>QTAPKTFTHPDTGIVFNTWSASDSQTKGGFTVGMALPSNALTTDATEFIGYLECSSAKNGANSGWCGVSLRGAMTNNLLITAWPSDGEVYTNLMFATGYAMPKNYAGDAKITQIASSVNATHFTLVFRCQNCLSWDQDGVTGGISTSNKGAQLGWVQAFPSPGNPTCPTQITLSQHDNGMGQWGAAFDSNIANPSYTAWAAKATKTVTGTCSGPVTTSIAATPVPTGVSFDYIVVGGGAGGIPVADKLSESGKSVLLIEKGFASTGEHGGTLKPEWLNNTSLTRFDVPGLCNQIWKDSDGIACSDTDQMAGCVLGGGTAINAGLWYKPYTKDWDYLFPSGWKGSDIAGATSRALSRIPGTTTPSQDGKRYLQQGFEVLANGLKASGWKEVDSLKDSEQKNRTFSHTSYMYINGERGGPLATYLVSAKKRSNFKLWLNTAVKRVIREGGHITGVEVEAFRNGGYSGIIPVTNTTGRVVLSAGTFGSAKILLRSGIGPKDQLEVVKASADGPTMVSNSSWIDLPVGHNLVDHTNTDTVIQHNNVTFYDFYKAWDNPNTTDMNLYLNGRSGIFAQAAPNIGPLFWEEITGADGIVRQLHWTARVEGSFETPDGYAMTMSQYLGRGATSRGRMTLSPTLNTVVSDLPYLKDPNDKAAVVQGIVNLQKALANVKGLTWAYPSANQTAADFVDKQPVTYQSRRSNHWMGTNKMGTDDGRSGGTAVVDTNTRVYGTDNLYVVDASIFPGVPTTNPTAYIVVAAEHAAAKILAQPANEAVPKWGWCGGPTYTGSQT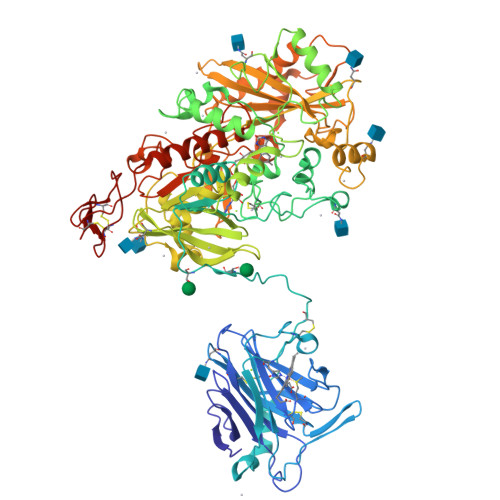CQAPYKCEKQNDWYWQCV[2x]> RPRLAPPQNVTLLSQNFSVYLTWLPGLGNPQDVTYFVAYQSSPTRRRWREVEECAGTKELLCSMMCLKKQDLYNKFKGRVRTVSPSSKSPWVESEYLDYLFEVEPAPPVLVLTQTEEILSANATYQLPPCMPPLDLKYEVAFWKE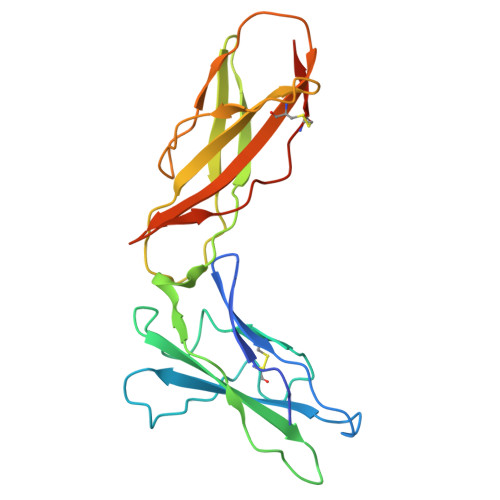GAGNKTLFPVTPHGQPVQITLQPAASEHHCLSARTIYTFSVPKYSKFSKPTCFLLEVPEANAAA> MAHHHHHHSSGLEVLFQMTISAQVIDTIVEWIDDNLHQPLRIDDIARHAGYSKWHLQRLFLQYKGESLGRYIRERKLLLAARDLRDTDQRVYDICL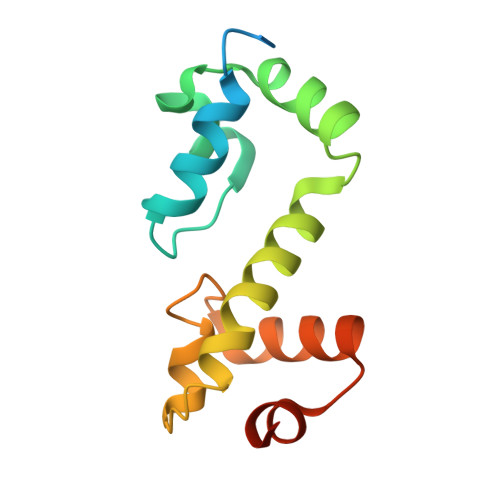KYGFDSQQTFTRVFTRTFNQPPGAYRKENHSRAH> H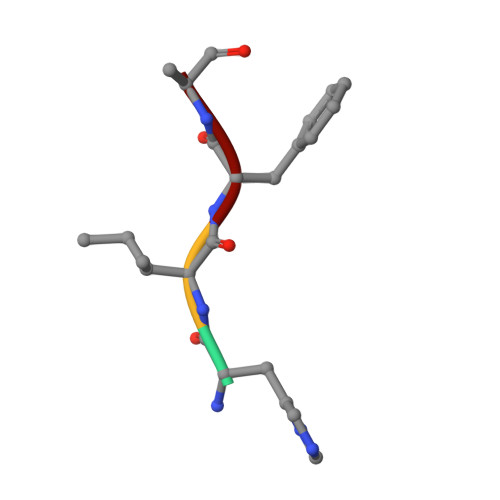IFS> MPGREILVLHVGQGGNQIGYNFWKTICEEHNIDIRSNQRKSVEEDKVDYKSVFLVEAPDGFHPRALFIDLEPLAVEFLVKEMKLGSFFSEDLMVLSYSGAHNVWSIGYQTGKKLIPVILEKIRDTMPETLQGFLIIHTLGGGTGSGFGSLLTETLKKEFPGKGVLNFSVLPSEVNDVTLAPYNTVLSLNHLSRFSDLVVLFDNTALIRIVKDQLNYPVIKQFSDLNFLIGRVMASITASLRFPGPLNMDLMEMAHNLVALPETKFIIPSVAPLTKEESEMSTELDLVERCFDPTHYMVNCSGQGKTISSVLMFRGNIAIENAFSIMTDIKSNVAFAPGVHPDLGLKYGICESAPVDFDKEVTLLSNNTIISEVFNRVLERFDSLFNRDWYTSD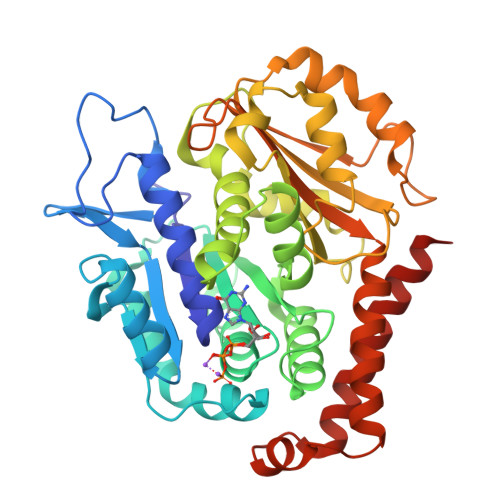YVNAGTSKSNLKEARDNFDRIIKIYKEIEGSQ>[2x]GMDNSEEKKLEALGAFEISRKMLALAQKNEKSNIFLNAGRGNPNWIQTLARLAFVRLVQFGVTESKLTINNGIMAGYINTDGIRERLFAFLDPDKNDEDKFLI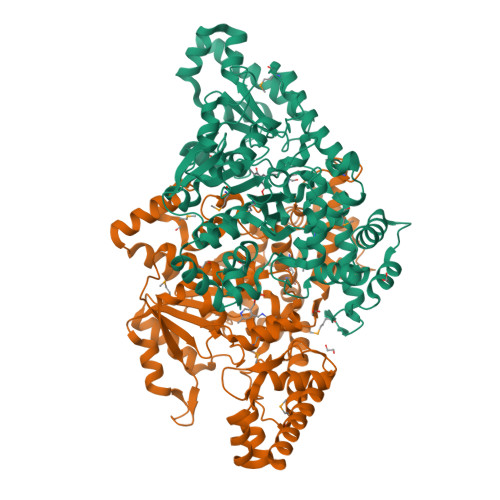DAVNYCHTELGLNRDKVVAEWVNGAVANNYPVPDRCLVNTEKIINYFLQELSYKDANLAEQTDLFPTEGGTAAIVYAFHSLAENHLLKKGDKIAINEPIFTPYLRIPELKDYELVEVDLHSYEKNDWEIEPNEIEKLKDPSIKALIVVNPTNPTSKEFDTNALNAIKQAVEKNPKLMIISDEVYGAFVPNFKSIYSVVPYNTMLVYSYSKLFGCTGWRLGVIALNEKNVFDDNIAHLDKVELRQLHKRYSSVVLDPDKMKFIDRLCADSRSIGLYHTAGLSTPQQIMEALFSMTHLLTSTNGGSDDPYIDIARKLVSERYDQLHDAMQAPKDETDTNTHYYSLIDIYRLAEKIYGKEFRDYLTNNFEQVDFLLKLAEKNGVVLVDGVGFGAKPGELRVSQANLPTEDYALIGKQVLELLKEYYEEFKQNN> GSHMSKSLKKLVEESREKNQPEVDMSDRGISNMLDVNGLFTLSHITQLVLSHNKLTMVPPNIAELKNLEVLNFFNNQIEELPTQISSLQKLKHLNLGMNRLNTLPRGFGSLPALEVLDLTYNNLSENSLPGNFFYLTTLRALYLSDN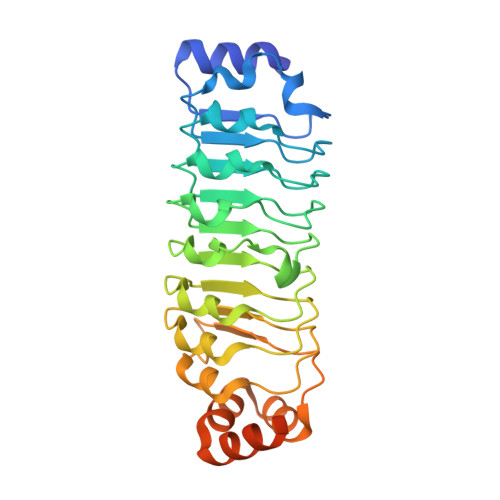DFEILPPDIGKLTKLQILSLRDNDLISLPKEIGELTQLKELHIQGNRLTVLPPELGNLDLTGQKQVFKAENNPWVTPIADQFQLGVSHVFEYIRSETYKYLYGRHMQANPEPPKKNNDKSKKISRKPLAAKNR> DSKKDISNVKSDLLYAYTITPYDYKDCRVNFSTTHTLNIDTQKYRGKDYYISSEMSYEASQKFKRDDHVDVFGLFYILNSHTGEYIYGGITPAQNNKVNHKLLGNLFISGESQQNLNNKIILEKDIVTFQEI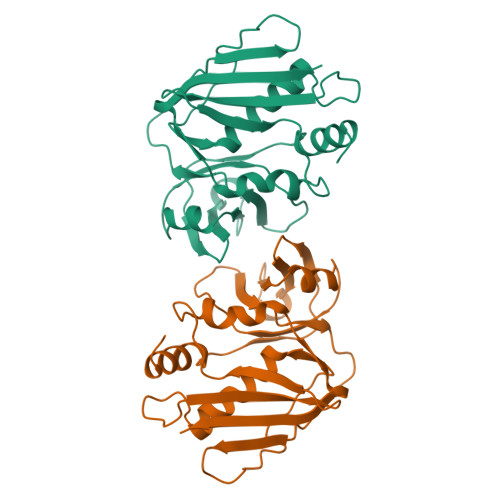DFKIRKYLMDNYKIYDATSPYVSGRIEIGTKDGKHEQIDLFDSPNEGTRSDIFAKYKDNRIINMKNFSHFDIYLEK> GSMVEATAQETDRPRFSFSIAAREGKARTGTIEMKRGVIRTPAFMPVGTAATVKALKPETVRATGADIILGNTYHLMLRPGAERIAKLGGLHSFMGWDRPILTDSGGYQVMSLSSLTKQSEEGVTFKSHLDGSRHMLSPERSIEIQHLLGSDIVMAFDESTPYPATPSRAASSMERSMRWAKRSRDAFDSRKEQAENAALFGIQQGSVFENLRQQSADALAEIGFDGYAVGGLAVGEGQDEMFRVLDFSVPMLPDDKPHYLMGVGKPDDIVGAVERGIDMFDSVLPTRSGRNGQAFTWDGPINIRNARFSEDLKPLDSECHCAVCQKWSRACIHALIRAGEILGAMLMTEHNIAFYQQLMQKIRDSISEGRFSQFAQDFRARYF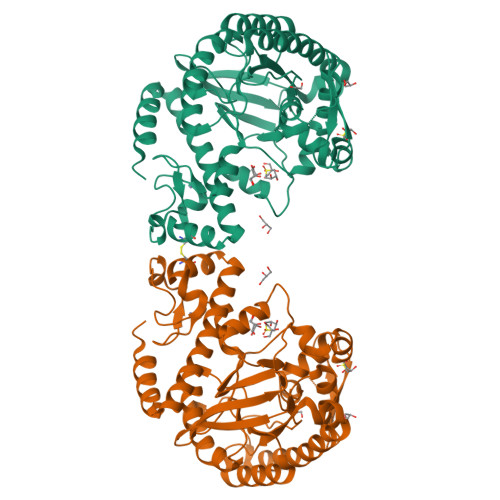ARNS> MALIQSDFAQGIRMTPVPDCAGDVTACRFDITLKNAPAAGDIIELGVLPGNAVPVEAILDVDDLDTGGAPTITLDVGIMSGPVGKNDPARTCGNELFAASTVGQAGGVVRATASSAFRIQKAEDHRSVGVKVAAGPA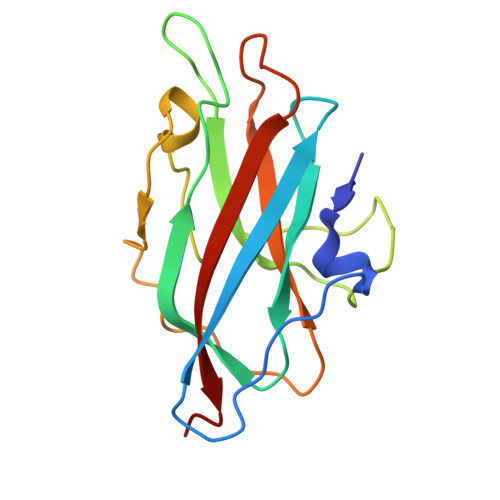TGAAGKTIALILFYVQGTSQ>[2x]EELQNKLEDVVIDRNLLILGKILGEGEFGSVMEGNLKQEDGTSLKVAVKTMKLDNSSQREIEEFLSEAACMKDFSHPNVIRLLGVCIEMSSQGIPKPMVILPFMKYGDLHTYLLYSRLETGPKHIPLQTLLKFMVDIALGMEYLSNRNFLHRDLAARNCMLRDDMTVCVADFGLSK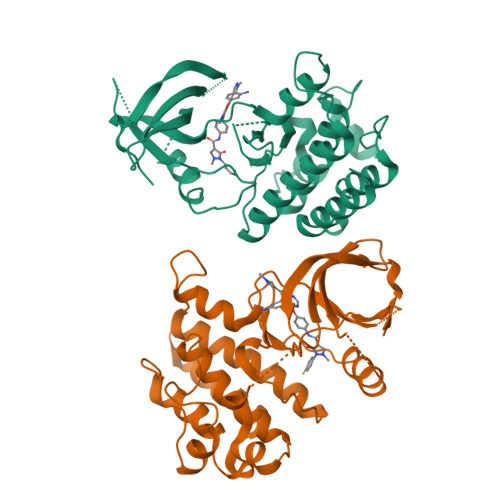KIYSGDYYRQGRIAKMPVKWIAIESLADRVYTSKSDVWAFGVTMWEIATRGMTPYPGVQNHEMYDYLLHGHRLKQPEDCLDELYEIMYSCWRTDPLDRPTFSVLRLQLEKLLESLPDV>MVANPEHYIKHPLQNRWALWFFKNDKSKTWQANLRLISKFDTVEDFWALYNHIQLSSNLMPGCDYSLFKDGIEPMWEDEKNKRGGRWLITLNKQQRRSDLDRFWLETLLCLIGESFDDYSDDVCGAVVNVRAKGDKIAIWTTECENREAVTHIGRVYKERLGLPPKIVIGYQSHADTATKSGSTTKNRFVV[2x];>XRYSRLQLLLLFRX[2x]

The eukaryotic translation initiation factor 4E (eIF4E) protein is a vital component of the cap-dependent mechanism for mRNA translation. It binds the 7-methylguanosine (m7G) cap structure present at the 5′ end of mRNA molecules and recruits it as part of the eIF4F assembly which also includes two other partner proteins, eIF4A and eIF4G, to the translational machinery for protein synthesis. We have used a structure-guided approach to rationally develop a set of hydrocarbon stapled-peptides with high binding affinities and residence times against the oncogenic eukaryotic translation initiation factor 4E (eIF4E) protein. Crystal structures of these peptides in complex with eIF4E show that they form specific interactions with a region on the protein-binding interface of eIF4E which is distinct from the other well-established canonical interactions.

The 10mer sTIP-12 stapled-peptide had only moderate binding affinity (KD of 397 nM) for eIF4E and thus we synthesized two derivatives of this peptide with their C-termini extended to investigate if the potential interaction with the patch can improve affinity. This included a 12mer peptide with “11FR12” addition and F10L substitution (sTIP-14), and a 13mer peptide with an i, i + 4 staple (sTIP-15) around the extended “10FQR13” sequence at the C-terminus. Phenylalanine and glutamine residues characterize distinct chemical properties which are complimentary to the targeted patch on eIF4E. It is interesting to observe that sTIP-14 and sTIP-15 respectively showed a 2-fold and a 7-fold improvement (KD of 195 nM and 54 nM respectively) in binding eIF4E; the latter is clearly comparable to other good binders reported in this study. The 2-fold improvement in the KD of sTIP-14 over sTIP-12 is primarily due to a 2-fold reduction in its rate of dissociation (koff: 0.058 s–1 and 0.14 s–1 respectively). The phenylalanine residue (F11) of the added “11FR12” sequence efficiently interacts with the patch on eIF4E by forming pi-stacking interactions with aromatic residues W73, Y76 and hydrophobic interactions with L131. The last arginine (R12) is exposed to the solvent and does not appear to form any specific interactions with the protein in the crystal structure. The bound-state conformations of sTIP-10 and sTIP-14 reveal that terminal modulation of their sequences results in interesting conformational properties of the peptides. sTIP-14 was optimized with regard to the positive chemical potential at the N-terminal end which is as critical as the conserved “YXXXXLφ” motif for the peptide to recognize and interact with eIF4E.2,6-dioxo-1,2,3,6-tetrahydropyridine-4-carboxylic acid | C6 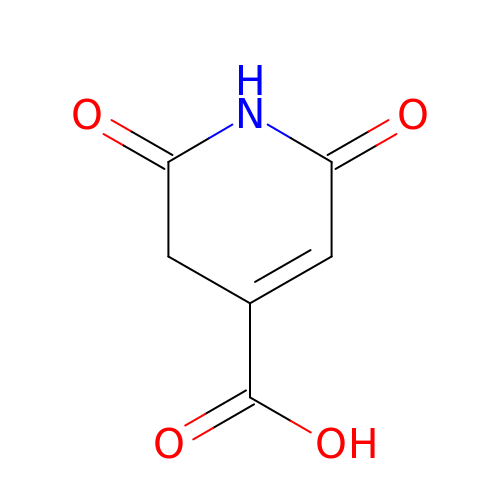H5 N O4 | RELAYXOQOWYDAT-UHFFFAOYSA-N>[4x]TSDNFFENELYSNYKFQGEVDQSIQRLSGSLQEKAKKVKYVPTAAWLAWSGATNEVARYLNEAGSKTVVFVLYMIPTRDCNAGGSNGGADNLSTYQGYVNSIYNTINQYPNSRIVMIIEPDTIGNLVTANNANCRNVHDMHKQALSYAISK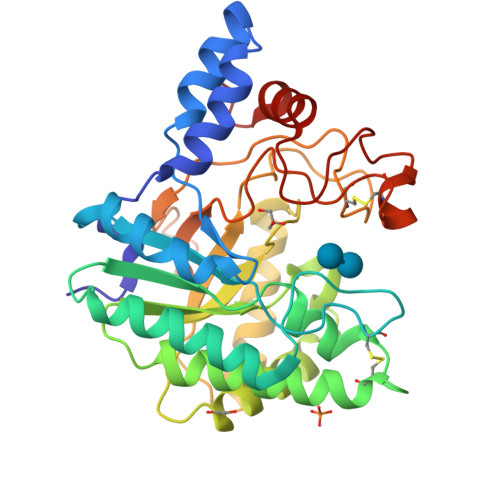FGTQKNVRVYLDAAHGGWLNSSADRTAEVIAEILRNAGNGKIRGISTNVSNYQPVYSEYQYHQNLNRALESRGVRGMKFIVDTSRNGRNPSSATWCNLKGAGLGARPQANPDPNMPLLDAYVWIKTPGESDSASSADPVCRNSDSLQGAPAAGSWFHDYFVMLLENANPPF>HHMFTGSIVAIVTPMDEKGNVCRASLKKLIDYHVASGTSAIVSVGTTGESATLNHDEHADVVMMTLDLADG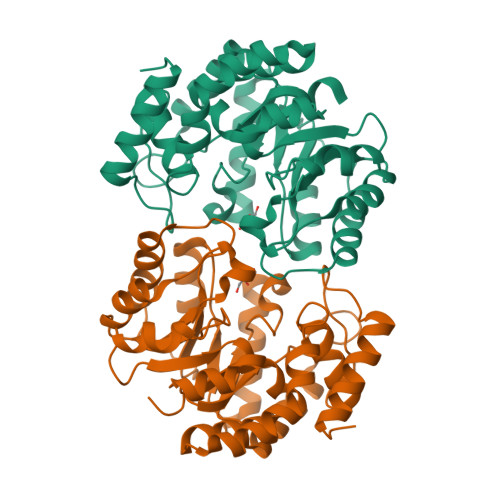RIPVIAGTGANATAEAISLTQRFNDSGIVGCLTVTPYYNRPSQEGLYQHFKAIAEHTDLPQILYNVPSRTGCDLLPETVGRLAKVKNIIGIXEATGNLTRVNQIKELVSDDFVLLSGDDASALDFMQLGGHGVISVTANVAARDMAQMCKLAAEGHFAEARVINQRLMPLHNKLFVEPNPIPVKWACKELGLVATDTLRLPMTPITDSGRETVRAALKHAGLL[8x]>[2x]MIIPALDLIGDTVVRVVRLHQGDYARQRDYGNDPLPRLQDYAAQG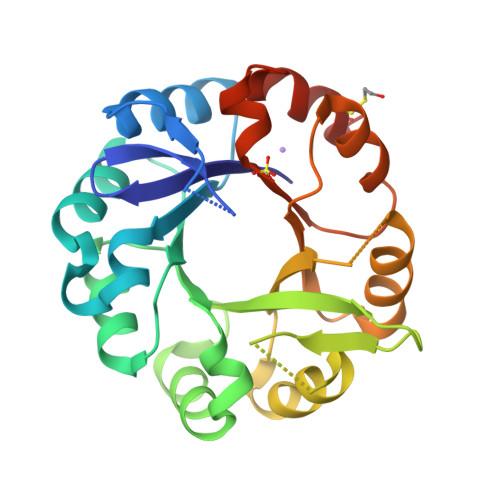AEVLHLVDLTGAKDPAKRQIPLIKTLVAGVNVPVQVGGGVRTEEDVAALLKAGVARVVIASTAVKSPDVVKGWFERFGAQALVLALDVRIDEHGTKQVAVSGWQENSGVSLEQLVETYLPVGLKHVLCTDISRDGTLAGSNVSLYEEVCARYPQIAFQSSGGIGDIDDIAALRGTGVRGVIVGRALLEGKFTVKEAIQCWQNVKGHHHHHH desferrioxamine 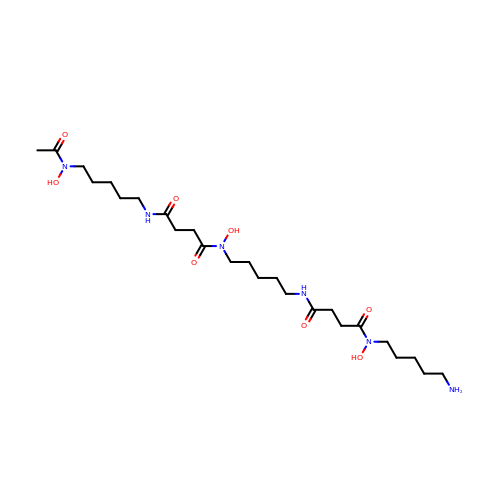B | C25 H48 N6 O8 | UBQYURCVBFRUQT-UHFFFAOYSA-N(1R,9S)-13-[(8-azanyl-3-methyl-[1,2,4]triazolo[4,3-a]pyridin-6-yl)carbonyl]-11,13-diazatricyclo[7.3.1.0^{2,7}]trideca-2,4,6-trien-10-one | C19 H18 N6 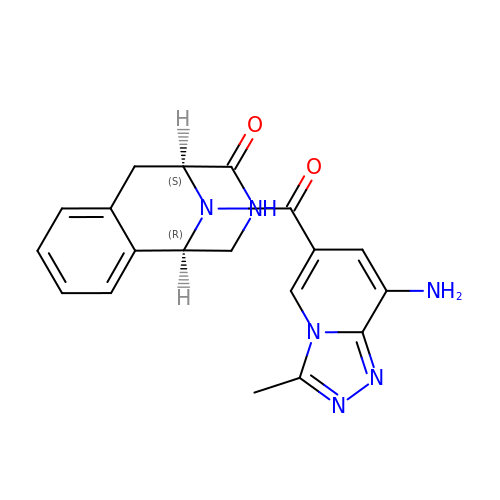O2 | MHYBWRVBBIRKIQ-HOTGVXAUSA-N Thioredoxins (TRX) are small globular proteins of about 100–110 residues, which are conserved in all living organisms. They participate in multiple critical redox-reactions via the reversible oxidation of the active site CXXC catalytic motif1. Two TRX forms were described in Escherichia coli, Trx1 and Trx22. The former, called EcTRX throughout this work, is a widely used experimental model for investigating the molecular basis of protein stability, folding and function.

However, in the E101G mutant, an interesting case of structural variability was observed. In this mutant, an extended, non-sequentially continuous region of the protein backbone presents two alternative traces for only one of two monomers found in the asymmetric unit. The widespread alternative-conformation region involves residues: (i) Asp10 to Val25 (including helix 1 and a half of strand β2) (ii) Thr77 to Val91 (comprising strands β4 and β5); and (iii) Ser95 to Leu107 (involving the complete CTH). Occupancies of these conformations equals 50%, and no clashes or packing defects result when alternatively occupied segments are assigned to different single-conformation models. The RMSD between these alternative conformations is 0.65 Å for the backbone atoms and it occurs without significant changes in the radius of gyration or total accessible surface area (data not shown). Structural differences between these alternative traces are explained mostly through rigid-body displacements of structural elements, as a result of changes in dihedral angles for the first and last residues of each segment. A well-preserved hydrogen bonding pattern is found in the CTH of E101G mutant, even though a Gly residue is highly destabilizing for the α-helical structure. Consistent with our previous report regarding an increase in enzyme activity when assayed using DiFTC-insulin12, the rate constant of E101G reacting with DiFTC-insulin was twice that of wild type EcTRX. Given that a negatively charged residue (Glu) is replaced by a neutral amino acid (Gly), we suspect that this difference in charge may alter the electrostatics of protein-protein interactions modifying in a subtle form the interaction with EcTPx, one of the natural targets of EcTRX, or with the non-natural substrate DiFICT-insulin, and concomitantly the EcTRX activity. The alternative conformation observed for the backbone of the E101G variant conform, to our knowledge, the widest region with alternative traces for the backbone reported to date.

>MSDKIIHLTDDSFDTDVLKADGAILVDFWAEWCGPCKMIAPILDEIADEYQGKLTVAKLNIDQNPGTAPKYGIRGIPTLLLFKNGEVAATKVGALSKGQLKGFLDANLA[2x]> HMGSDTDERCA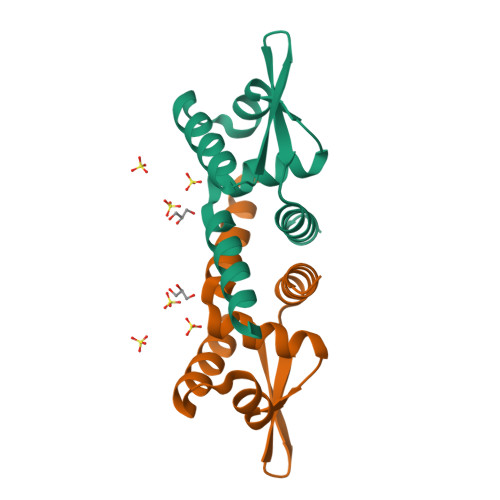ALDAEEMATRARAASNLLKALAHEGRLMIMCYLASGEKSVTELETRLSTRQAAVSQQLARLRLEGLVQSRREGKTIYYSLSDPRAARVVQTVYEQFCSGD>[2x]AEAESALEYAQQALEKAQL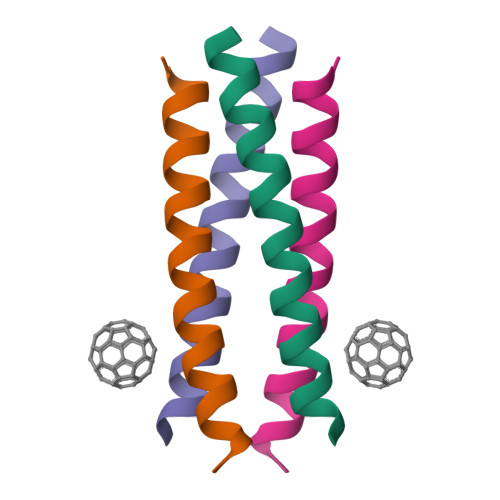ALQAARQALKA> MHHHHHHVTAELKPVTISGGGFISGLVAHPTEKDLIYARTDIGGTYRWNAAKWEWEPITDFIINNALAGNGANLLGTESIALDPHNPDRLYLAQGDYVQWDPWAAFLVSDDRGKTFKQYRSPVPMGAN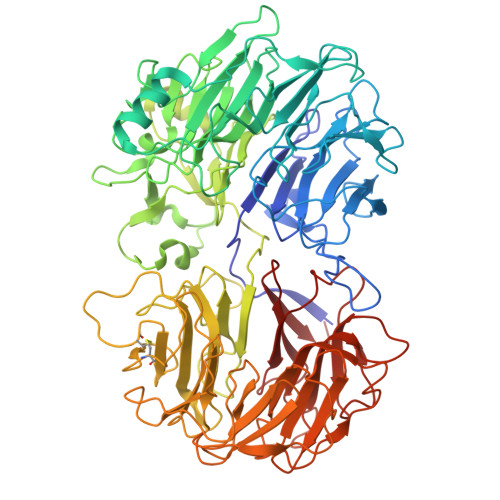DMGRNGGERLAVNPHWTDELWFGSRTQGLWRSTDRAQTWSRMNQLPDSSTYGIGIISVIFDPKNVGTAYVASHAVGGLWVTWDGGANWSQVGGQPTQWSDWTKSIVAASGTAIQSSGPLPIKIALGKNGRLYITYSDAPGPWGVLYGEVWSYDPTNGNWKHITPSREGANTYPAPTGNKKVVPGGWNGISVGNGDTVVVSTLDANGEDSVYLSRDAGNSWKDLGKLTTPAGAGGNSQKESDAKLRNGTPLPWLSFQNRGSGIVGFGWWLAAILLDPFSDRLLYGTGAVIWATDAVSRADSNQAPSWYINTEGIEETAILVLKSPPAGPAHLFSGMYDLGGMRHDDFSVPQPMYSKPTFSSTDGLDFAGRAANVLARVGRNDHPDAGVAGCTQGAYTTNSGDSWTLFQTCVPSLEVGNGGTIAVGADGKTFVWSPSKADGKGPYTSSDYGKTWTAPSGLSKQTTGIAADRVQANTFYVYVEGDFFVSTDGGKSYTKKGNGLPCCWTYTGTPVTSNLRAGELWVSVKGVGIYHSTDFGNTFTALAGSGSSLNPAVFSIGAPQTPNATETLFLWGIPSASQPEGLYMSTDNGGLWTRLNDDAHNYGGATVISGDPRIYGRVYIGMNGRGIICAQALGT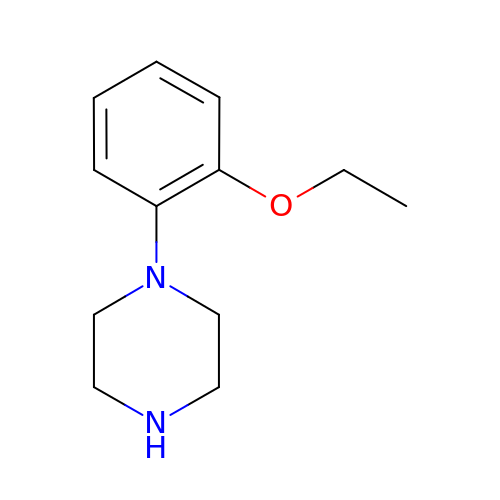1-(2-ethoxyphenyl)piperazine | C12 H18 N2 O | FBQIUSDQWOLCNY-UHFFFAOYSA-N> TVFRQENVDDYYDTGEELGSGQFAVVKKCREKSTGLQYAAKFIKKRRTKSSRRGVSREDIEREVSILKEIQHPNVITLHEVYENKTDVILILE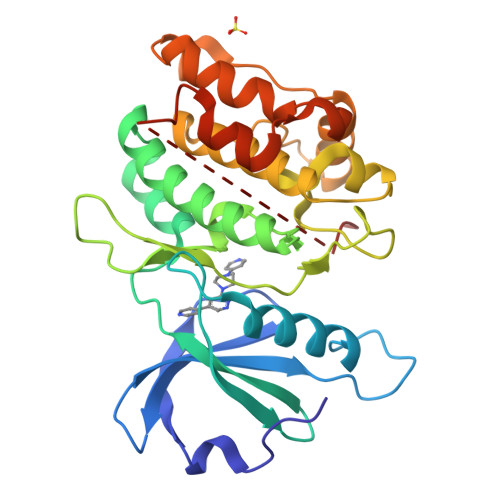LVAGGELFDFLAEKESLTEEEATEFLKQILNGVYYLHSLQIAHFDLKPENIMLLDRNVPKPRIKIIDFGLAHKIDFGNEFKNIFGTPEFVAPEIVNYEPLGLEADMWSIGVITYILLSGASPFLGDTKQETLANVSAVNYEFEDEYFSNTSALAKDFIRRLLVKDPKKRMTIQDSLQHPWIKPKDTQQALSSAWSHPQFE> GHMKKILVLGGAHIDRRGMIETETAPGASNPGSWMEEAGGGGFNAARNLSRLGFEVRIIAPRGGDVTGEVVAEAARQAGVEDTPFTFLDRRTPSYTAILERDGNLVIALADMDLYKLFTPRRLKVRAVREAIIASDFLLCDANLPEDTLTALGLIARACEKPLAAIAISPAKAVKLKAALGDIDILFMNEAEARALTGETAENVRDWPNILRKAGLSGGVVTRGASEVVAFNGTEKAILHPPLIREVKDVTGAGDAMASGYLAAIAEGKTIREALRQGA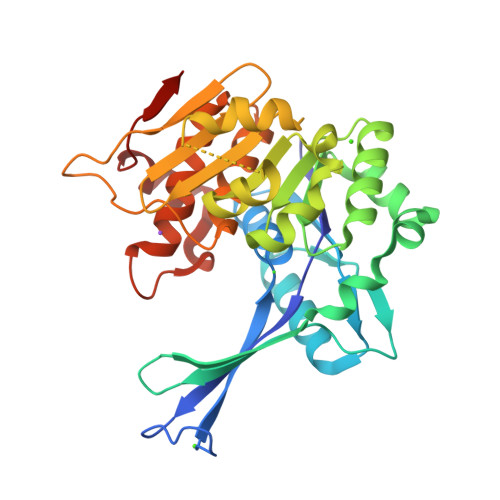AAAAITVQSSFATSQDLSKDSVEAMLGLVPQAEMLAGS2-chloro-N-{2-[4-chloro-3-(3-chloro-5-cyanophenoxy)phenyl]ethyl}acetamide 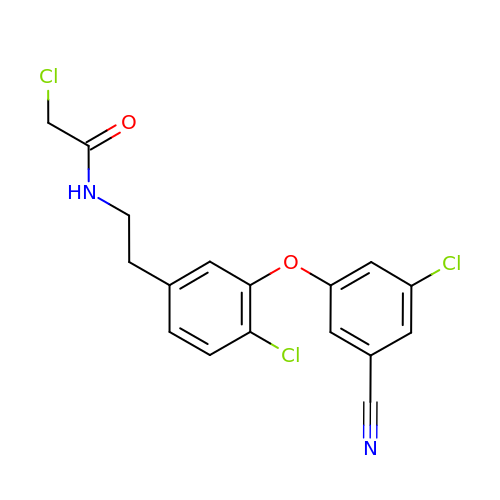| C17 H13 Cl3 N2 O2 | FODVGONJGOTOHH-UHFFFAOYSA-N>[4x]SNAPTLYEKIQQANEEAVTRIIQSKPILVGFDKAINVMPDMTE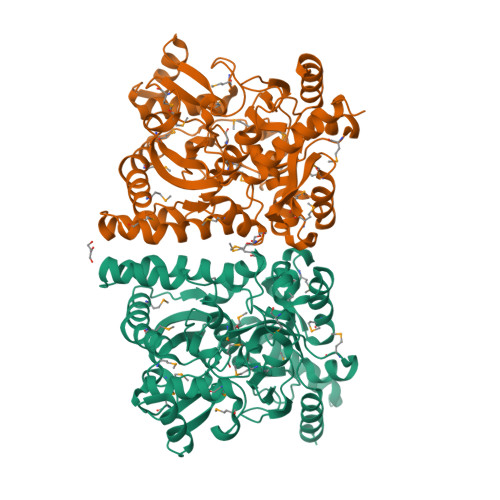TTILHAGPPITYENMCGPMKGAVQGALVFEGLAKDLADADRVARSGAITFSPCHEHDAVGSMAGVTSPNMYVHIIKNETYGNTAFTNLSEQLAKVLRFGANDQSVVDRLIWMRDVLGPLLHDAMTFCPEGIDLRLMLSQALHMGDECHNRNVAGSTLLVQALTPYMVQTDFSREQLKEVFEFLGSSDYFSGPTWMGAAKCALDAGHNVENSTIVTTMCRNGVEFGIRVSGIGGNHWFTGPAQRVIGPMFAGYTQEDAGLDMGDSAITETYGVGGFAMAAAPAIVPLVGGTVAEALNYSKEMLEITTKENPNVTIPVLDFMGIPTGIDVLKVLETGMLPVINTAIAHKEPGIGMIGAGLTNPPANVFNEALKALVATIN> SRVLLALHDRAPQLKISDDRLTVVGEKGYSMVRASHGVRKGAWYFEITVDEMPPDTAARLGWSQPLGNLQAPLGYDKFSYSWRSKKGTKFHQSIGKHYSSGYGQGDVLGF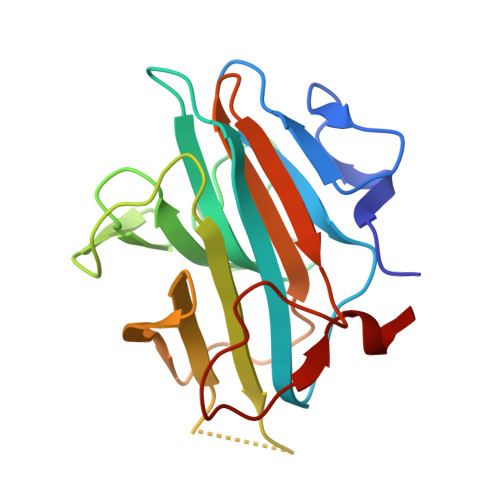YINLPEDTISGRGSSEIIFYKNGVNQGVAYKDIFEGVYFPAISLYKSCTVSINFGPCFKYPPKDLTYRPMSDMG>[2x]METIQELILSEENKTNIAVLNLGTNDRRNAVLILETALHLVEKY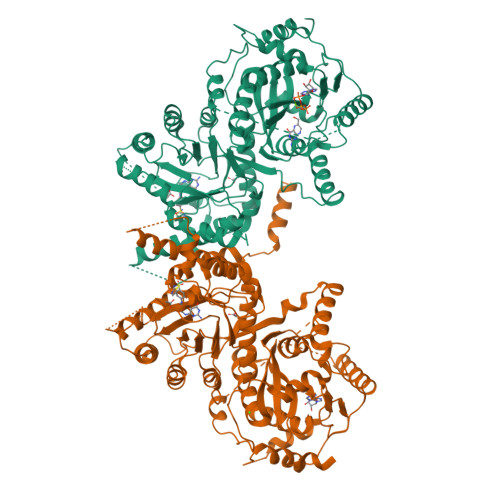LGKIINTSYLYETVPEYIVLDKKESCEKINKDCRIYDVNYINELMQNLEESKYEENKELIDKCEEYETFLKNGKVDNSILKEVNVENYLLECNNIIVKNDEIMKNNLSKYKDKYYTSYFYNLTVVVKTFVNDPLSMLVVIKYIEELMKRENVKEKEKFENRIIDIDILFFNDFTIFMKNIKLEKNMIYKILSKYIHLERDIKNGNDNMSKVNMDKDINLNNNNNIKKKNNNDIDCDCVDQKMNNHVNNKNYINSFRDPQEIINNMVDNIEFLSIPHVYTTHRYSILLCLNDMIPEYKHNVLNNTIRCLYNKYVSRMKEQYNINIKENNKRIYVLKDRISYLKEKTNIVGILNVNYDSFSDGGIFVEPKRAVQRMFEMINEGASVIDIGGESFGPFVIPNPKISERDLVVPVLQLFQKEWNDIKNKIVKCDAKPIISIDTINYNVFKECVDNDLVDILNDISACTNNPEIIKLLKKKNKFYSVVLMHKRGNPHTMDKLTNYDNLVYDIKNYLEQRLNFLVLNGIPRYRILFDIGLGFAKKHDQSIKLLQNIHVYDEYPLFIGYSRKRFITHCMNDQNVVINTQQKLHDEQQNENKNIVDKSHNWMFQMNYMRKDKDQLLYQKNICGGLAIASYSYYKKVDLIRVHDVLETKSVLDVLTKIDQVKDPNSSSVDKLAAALEHHHHHH> 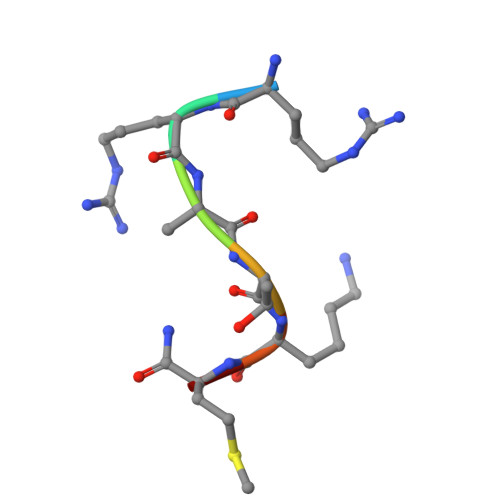RRATKMX>[4x]IINGEDCSPHSQPWQAALVMENELFCSGVLVHPQWVLSAAHCFQNSYTIGLGLHSLEADQEPGSQM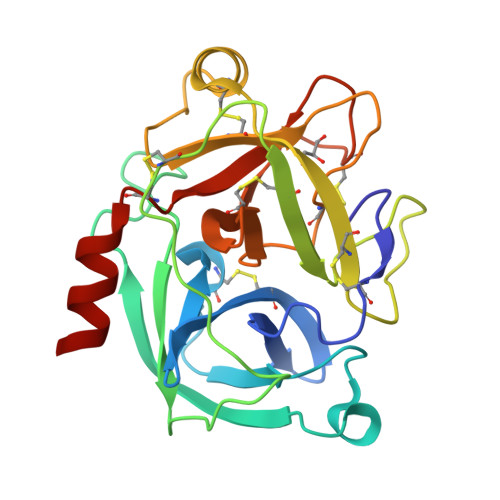VEASLSVRHPEYNRPLLANDLMLIKLDESVSESDTIRSISIASQCPTAGNSCLVSGWGLLANGRMPTVLQCVNVSVVSEEVCSKLYDPLYHPSMFCAGGGQDQKDSCNGDSGGPLICNGYLQGLVSFGKAPCGQVGVPGVYTNLCKFTEWIEKTVQAS>[2x]MRQATVYIDRQALQYNLNRVKQLAANSKIVS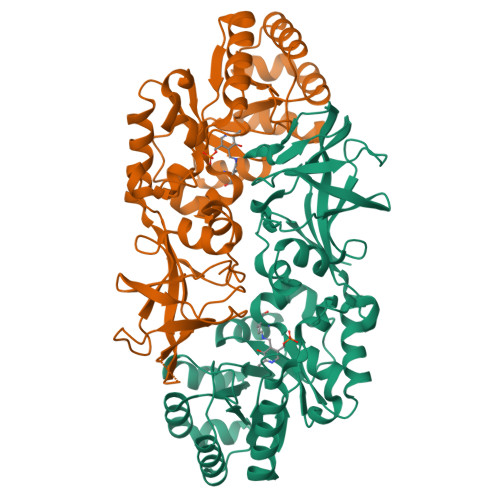MVKANAYGHGVKDCLAALNASDAFGVACLQEGLEIRELGFEQPVTLIEGVFSEDEMPVAIEQKFECVIHHQQQFEWLIKHKQAYIAQGLKVWVKLNSGMNRLGFKDPEIIEVIKTLKSEGFTCVLAMHFANADVDHPLNEQQKQQFLHIKETCDPILASCCNSAAIFKWPELNFDYVRPGIMLYGASPFADKTVHDLDLKPVMTFTAEIIALNHIEAGEHVGYGSTFCAQQAMDIAIVSIGYGDGYPRAYVKQNFVAIDGKLCPVVGRVSMDMIAIDVTNTQVKLGTQVELWGNHRLVDDVAEANGTIGYELLCRLSSRPVRQGT> LRQSSLLCFSTFALNPETSRAPHGPPRGLINRYISMGLPPWAAWCNRVNRHALYRMSDVSPRSFLPKAPHEMDVIWMNERVRERVRTSRQVQHVYRQLKYPFVKTGIHYSDTLDHWVQVPMVEAAMFEIEKDGGFDNFILKRSGPELRSTYGERIRRHLLVRQKETQKNFVLDQQAKALAEVTQAELMKATSEE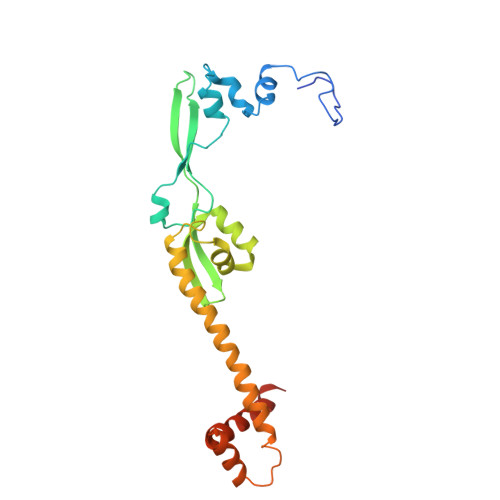ELDAVLAKYGMDAEEFKRLMAKRVMEQRKSVAAAGLRSK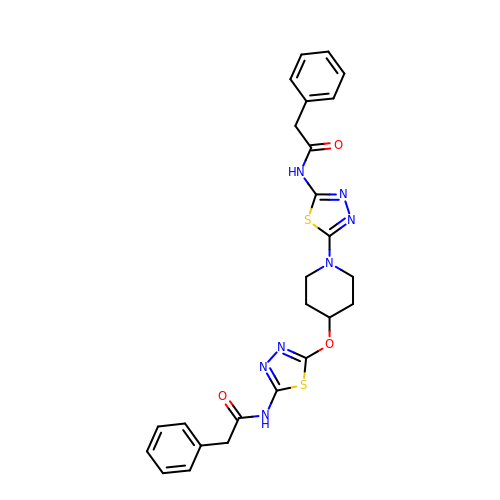2-phenyl-N-{5-[4-({5-[(phenylacetyl)amino]-1,3,4-thiadiazol-2-yl}oxy)piperidin-1-yl]-1,3,4-thiadiazol-2-yl}acetamide | C25 H25 N7 O3 S2 | BAGWZESOKRULGY-UHFFFAOYSA-N> GNITDIKVSSLPNKQKIVKVSFDKEIVNPTGFVTSSPARIALDFEQTGISMDQQVLEYADPLLSKISAAQNSSRARLVLNLNKPGQYNTEVRGNKVWIFINESDDTVSAPARPAVKAAPAAPAKQQAAAPSTKSAVSVSEPFTPAKQQAAAPFTESVVSVSAPFSPAKQQAAASAKQQAAAPAKQQAAAPAKQQAAAPAKQTNIDFRKDGKNAGIIELAALGFAGQPDISQQHDHIIVTLKNHTLPTTLQRSLDVADFKTPVQKVTLKRLNNDTQLIITTAGNWELVNKSAAPGYFTFQVLPKKQNLESGGVNNAPKTFTGRKI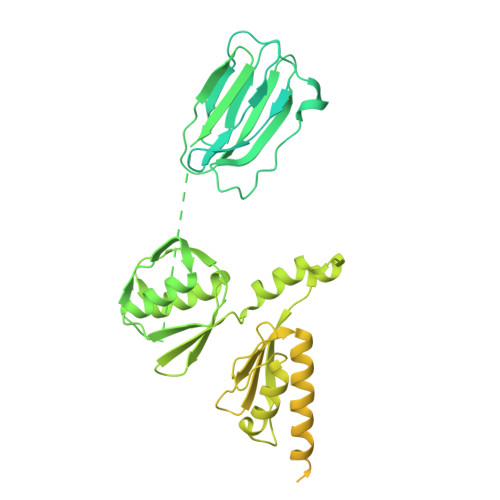SLDFQDVEIRTILQILAKESGMNIVASDSVNGKMTLSLKDVPWDQALDLVMQARNLDMRQQGNIVNIAPRDELLAKDKAFLQAEKDIADLGALYSQNFQLKYKNVEEFRSILRLDNADTTGNRNTLISGRGSVLIDPATNTLIVTDTRSVIEKFRKLIDELDVPAQQVMIEARIVEAADGFSRDLGVKFGATGKKKLKNDTSAFGWGVNSGFGGDDKWGAETKINLPITAAANSISLVRAISSGALNLELSASESLSKTKTLANPRVLTQNRKEAKIESGYEIPFTVTSIANGGSSTNTELKKAVLGLTVTPNITPDGQIIMTVKINKDSPAQCASGNQTILCISTKNLNTQAMVENGGTLIVGGIYEEDNGNTLTKVPLLGDIPVIGNLFKTRGKKTDRRELLIFITPRIMGTAGNSLRY>[4x]NVAPKFLANMTSVILPEDLPVGAQAFWLVAEDQDNDPLTYGMSGPNAYFFAVTPKTGEVKLASALDYETLYTFKVTISVSDPYIQVQREMLVIVEDRNDNAPVFQNTAFSTSINETLPVGSVVFSVLAVDKDMGSAGMVVYSIEKVIPSTGDSEHLFRILANGSIVLNGSLSYNNKSAFYQLELKACDLGGMYHNTFTIQCSLPVFLSISVVDQPDLDPQTVPRARDPPVGGHHHHHH

Enterocytes are specialized epithelial cells lining the luminal surface of the small intestine that build densely packed arrays of microvilli known as brush borders. These microvilli drive nutrient absorption and are arranged in a hexagonal pattern maintained by intermicrovillar links formed by 2 nonclassical members of the cadherin superfamily of calcium-dependent cell adhesion proteins: protocadherin-24 (PCDH24, also known as CDHR2) and the mucin-like protocadherin (CDHR5). PCDH24 belongs to the Cr-2 subfamily and has 9 EC repeats, a membrane adjacent domain (MAD10), a transmembrane domain, and a C-terminal cytoplasmic domain. PCDH24 is most similar to CDH23, having the residues and elongated N-terminal β-strand that are predicted to favor the formation of an atypical calcium-binding site at its tip. Here, we present X-ray crystal structures of the PCDH24 and CDHR5 extracellular tips and analyze their species-specific features relevant for adhesive interactions.

As expected, all EC repeats in all 3 PCDH24 structures adopt the typical 7 β-strand Greek-key fold seen in extracellular domains of cadherin proteins, with β-strands labeled A to G for each repeat. The crystallographic packings observed for the hs and mm PCDH24 structures show various interfaces that further highlight differences across species. Remarkably, there are 2 sets of potential antiparallel trans dimers. To probe the most promising trans interface observed in our human PCDH24 structures and to understand the different modes of adhesion observed in our bead aggregation assays, we introduced mutations into hs PCDH24 EC1-2Fc and EC1-3Fc fragments and tested their adhesive properties. Unexpectedly, bead aggregation experiments using hs PCDH24 EC1-2Fc p.Y67A and hs PCDH24 EC1-3Fc p.Y67A showed larger calcium-dependent aggregates than when using the wild-type protein fragments. In contrast, bead aggregation experiments using hs PCDH24 EC1-2Fc p.Y71A did not show aggregation with results similar to EDTA controls, while the size of the aggregates mediated by hs PCDH24 EC1-3Fc p.Y71A were markedly reduced when compared to those mediated by the wild-type protein. Likely, the p.Y67A mutation introduces some flexibility into the linker region that strengthens the π–π interaction between p.Y71 residues from adjacent monomers, while the p.Y71A mutation impairs the formation of an adhesive interface that is essential for bead aggregation mediated by hs PCDH24 EC1-2Fc and important for the larger bead aggregates mediated by hs PCDH24 EC1-3Fc. The tyrosine residue in the human protein (p.Y71), important for trans homophilic adhesion as suggested by our structure and bead aggregation assays, is not conserved, and it is switched to a smaller proline (p.P71) in the mouse protein.> MGSSHHHHHHSSGLVPRGSHVANTMASPNTPAPPNAAASPNPSDSPNPSDSPNPPASPNIEAILASYAGFRDRDIEGILSGMHPDVEWVHPEGMGKYGLGGTKLGHAGIKEFLAHVPTVLGGMRLAPREFIEQGDRVVVFGTREVTSLRGTTATLDFVHSW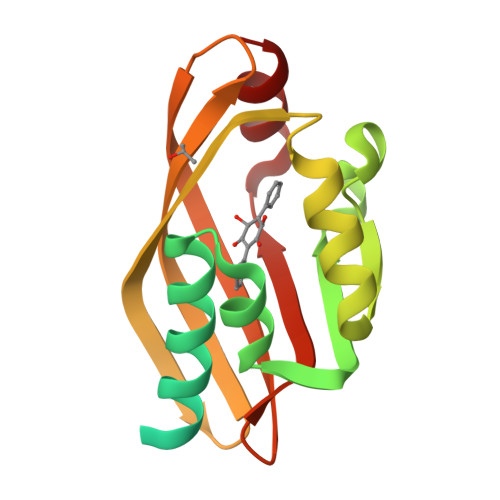TMRDGKATRMEDIFDTVAFHELIES> DTVGRPLPHLAAAMQASGEAVYCDDIPRYENELFLRLVTSTRAHAKIKSIDVSEAQKVPGFVCFLSADDIPGSNETGLFNDETVFAKDTVTCVGHIIGAVVADTPEHAERAAHVVKVTYEDLPAIITIEDAIKNNSFYGSELKIEKGDLKKGFSEADNVVSGELYIGGQDHFYLETHCTIAIPKGEEGEMELFVSTQNAMKTQSFVAKMLGVPVNRILVRVKRMGGGFGGKETRSTLVSVAVALAAYKTGHPVRCMLDRNEDMLITGGRHPFLARYKVGFMKTGTIVALEVDHYSNAGNSRDLSHSIMERALFHMDNCYKIPNIRGTGRLCKTNLSSNTAFRGFGGPQALFIAENWMSEVAVTCGLPAEEVRWKNMYKEGDLTHFNQRLEGFSVPRCWDECLKSSQYYARK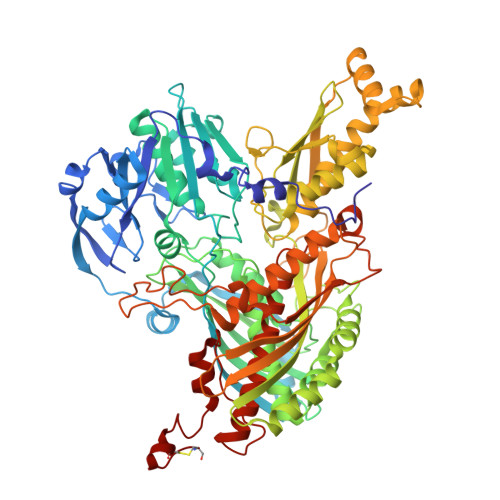SEVDKFNKENCWKKRGLCIIPTKFGISFTVPFLNQAGALIHVYTDGSVLVSHGGTEMGQGLHTKMVQVASKALKIPISKIYISETSTNTVPNSSPTAASVSTDIYGQAVYEACQTILKRLEPFKKKNPDGSWEDWVMAAYQDRVSLSTTGFYRTPNLGYSFETNSGNAFHYFTYGVACSEVEIDCLTGDHKNLRTDIVMDVGSSLNPAIDIGQVEGAFVQGLGLFTLEELHYSPEGSLHTRGPSTYKIPAFGSIPTEFRVSLLRDCPNKKAIYASKAVGEPPLFLGASVFFAIKDAIRAARAQHTNNNTKELFRLDSPATPEKIRNACVDKFTTLCVTGAPGNC> ATDATSLATDKDKLSYSIGADLGKNFKNQGIDVNPEAMAKGMQDAMSGAQLALTEQQMKDVLNKFQKDLMAKRTAEFNKKADENKVKGEAFLTENKNKPGVVVLPSGLQYKVINSGNGVKPGKSDTVTVEYTGRLIDGTVFDSTEKTGKPATFQVSQVIPGWTEALQLMPA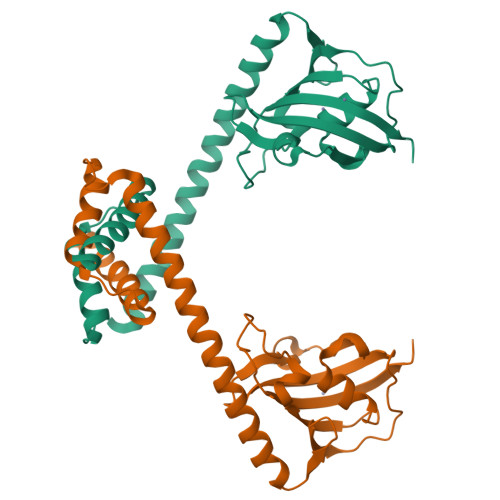GSTWEIYVPSGLAYGPRSVGGPIGPNETLIFKIHLISVKKSS> EMAKPVLPDLSGYTTEAALKKIARNKPGKITVARMMEETGLKEFIGGDNKMAEWVVRQKGIPQAIMISDGYVNLQDLVKKVPKQFLSEVSPGVYVARLPILVKETGIFEIDSKTKELRLSQEKGSFIVSEGKMLITNTSVNAWSETRNGLAAYRTPDEFRPFVLTWGGSQTWIAKTKMASMGYNQSKSYGVSISQYNPNTAKVLKRGEPTGWIIDSEFADMWYGFYCYETRDFVVKGNTYRDNIVYGIDPHDRSHGLIIAENDVYGTKKKHGIIISREVDNSFIFRNKSHNNKLSGVVLDRNSVGNIVAYNEIYQNHTDGITLYESGNNLLWGNRVIANRRHGIRVRNSVNIKLYENVAMANGLMGVYGHIKDLNDTDRDIELDPFD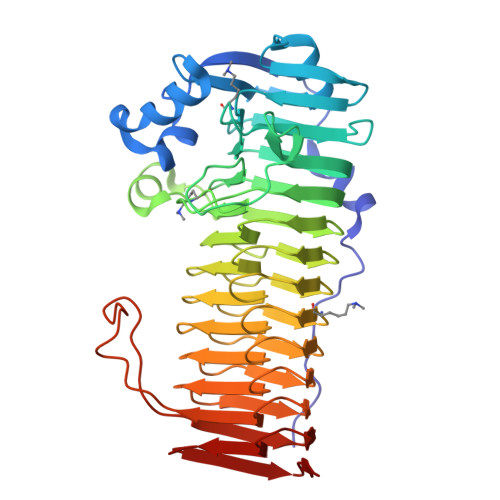AQVSLIMVGGELSSNGSGPLSIDSPLSVELYRVSML> MDHSITASYYDTTQQLSLLKHVLSEDKRPIAFIIAAGCPVSIRHNDAPLIPDVAGLTRKISDSFGGNPDSLLMKIIQNLKTTIPNPTIEDILSYIRLLQQIPMSGKIHDVENSVINALEESICELIEEEVNVDLPGNATPYH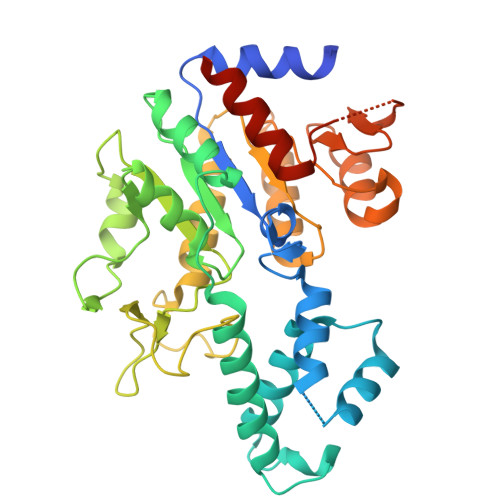KIAAWINSINREHQVEIFTTNYDLLMEQALEELNVPYFDGFVGSKRAFFDIRTIEENKLPSRWSKLWKLHGSINWQLDKQTQTIWRGTPSKGCSLIHPSHLKYDQSRKMPYLVMMDQLKLFLNQPSAILITCGYSYKDQHINEVLSQGLQTNPNALIYGLQYDVLENYQEAKDMALKRSNLILLAKDRAIIGKKEGEWKPDPQSSQDNDPLLFFKLGDFQHLASFLEEISQYDWSKQND> GDRVADMIESSIGNSVSRALTQALPAPTGQNTQVSSHRLDTGEVPALQAAEIGASSNTSDESMIETRCVLNSHSTAETTLDSFFSRAGLVGEI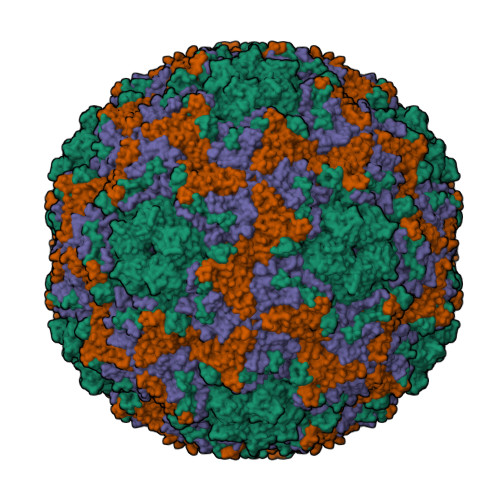DLPLEGTTNPNGYANWDIDITGCAQMRRKVELFTYMRFDAEFTFVACTPTGQVVPQLLQYMFVPPGAPIPESRESLAWQTATNPSVFVKLTDPPAQVSVPFMSPASAYQWFYDGYPTFGEHKQEKDLEYGACPNNMMGTFSVRTVGSSKSKYALVVRIYMRMKHVRAWIPRPMRNQNYLFKANPNYAGDSIKPTGTSRNAITTL;> MGSQVSTQRSGSHENSNSATEGSTINYTTINYYKDSYAATAGKQSLKQDPDKFANPVKDVFTEMAAPLKSPSAEACGYSDRVAQLTIGNSTITTQEAANIIVGYGEWPSYCSDDDATAVDKPTRPDVSVNRFYTLDTKLWEKSSKGWYWKFPDVLTETGVFGQNAQFHYLYRSGFCIHVQCNASKFHQGALLVAILPEYVIGTVAGGTGTEDSHPPYIQTQPGADGFELQHPYVLDAGIPISQLTVCPHQWINLRTNNCATIIVPYMNTLPFDSALNHCNFGLLVVPISPLDFDQGATPVIPITITLAPMCSEFAGLRQAVTQ;> GFPTELKPGTNQFLTTDDGVSAPILPNFHPTPCIHIPGEVRNLLELCQVETILEVNNVPTNATSLMERLRFPVSAQAGKGELCAVFRADPGRDGPWQSTMLGQLCGYYTQWSGSLEVTFMFTGSFMATGKMLIAYTPPGGPLPKDRATAMLGTHVIWDFGLQSSVTLVIPWISNTHYRAHARDGVFDYYTTGLVSIWYQTNYVVPIGAPNTAYIIALAAAQKNFTMKLCKDTSHMLQTASIQ>[3x]MTKRVRLSDSFNPVYPYEDESTSQHPFINPGFISPNGFTQSPNGVLTLKCLTPLTTTGGSLQLKVGGGLTVDDTNGFLKENISATTPLVKTGHSIGLPLGAGLGTNENKLCIKLGQGLTFNSNNICIDDNINTLWTGVNPTEANCQIMNSSESNDCKLILTLVKTGALVTAFVYVIGVSNNFNMLTTHRNINFTAELFFDSTGNLLTRLSSLKTPLNHKSGQNMATGAITNAKGFMPSTTAYPFNDNSREKENYIYGTCYYTASDRTAFPIDISVMLNRRAINDETSYCIRITWSWNTGDAPEVQTSATTLVTSPFTFYYIREDD;>MARSPGRAYALLLLLICFNVGSGLHLQVLSTRNENKLLPKHPHLVRQKRAWITAPVALREGEDLSKKNPIAKIHSDLAEERGLKITYKYTGKGITEPPFGIFVFNKDTGELNVTSILDREETPFFLLTGYALDARGNNVEKPLELRIKVLDINDNEPVFTQDVFVGSVEELSAAHTLVMKINATDADEPNTLNSKISYRIVSLEPAYPPVFYLNKDTGEIYTTSVTLDREEHSSYTLTVEARDGNGEVTDKPVKQAQVQIRILDVNDNIPVVENKVLEGMVEENQVNVEVTRIKVFDADEIGSDNWLANFTFASGNEGGYFHIETDAQTNEGIVTLIKEVDYEEMKNLDFSVIVANKAAFHKSIRSKYKPTPIPIKVKVKNVKEGIHFKSSVISIYVSESMDRSSKGQIIGNFQAFDEDTGLPAHARYVKLEDRDNWISVDSVTSEIKLAKLPDFESRYVQNGTYTVKIVAISEDYPRKTITGTVLINVEDINDNCPTLIEPVQTICHDAEYVNVTAEDLDGHPNSGPFSFSVIDKPPGMAEKWKIARQESTSVLLQQSEKKLGRSEIQFLISDNQGFSCPEKQVLTLTVCECLHGSGCREAQHDSYVGLGPAAIALMILAFLLLLLVPLLLLMCHCGKGAKGFTPIPGTIEMLHPWNNEG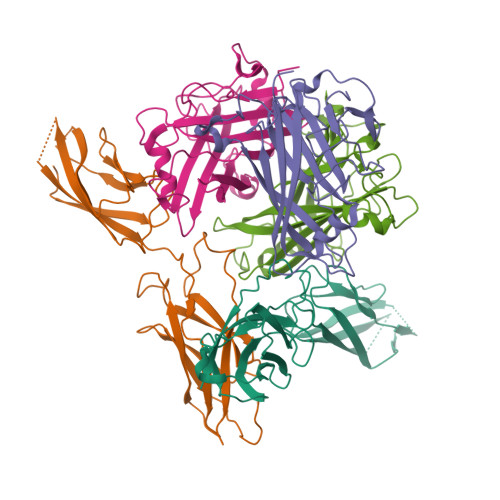APPEDKVVPSFLPVDQGGSLVGRNGVGGMAKEATMKGSSSASIVKGQHEMSEMDGRWEEHRSLLSGRATQFTGATGAIMTTETTKTARATGASRDMAGAQAAAVALNEEFLRNYFTDKAASYTEEDENHTAKDCLLVYSQEETESLNASIGCCSFIEGELDDRFLDDLGLKFKTLAEVCLGQKIDINKEIEQRQKPATETSMNTASHSLCEQTMVNSENTYSSGSSFPVPKSLQEANAEKVTQEIVTERSVSSRQAQKVATPLPDPMASRNVIATETSYVTGSTMPPTTVILGPSQPQSLIVTERVYAPASTLVDQPYANEGTVVVTERVIQPHGGGSNPLEGTQHLQDVPYVMVRERESFLAPSSGVQPTLAMPNIAVGQNVTVTERVLAPASTLQSSYQIPTENSMTARNTTVSGAGVPGPLPDFGLEESGHSNSTITTSSTRVTKHSTVQHSYS[2x]>[2x]MATLICGSIAYDNIMTFEGRFREHI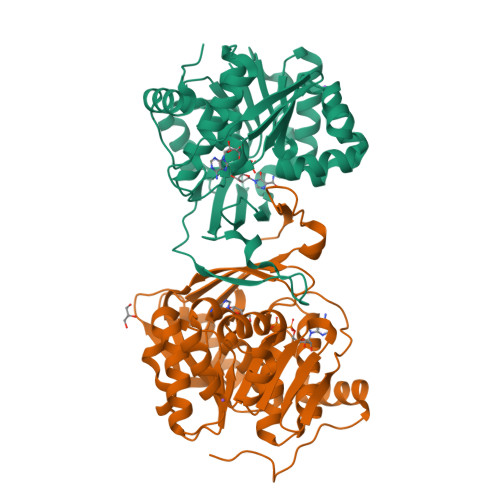LPDQVHLINLSFLVPTMRREFGGCAGNIAYALNLLGGDARMMGTLGAVDAQPYLDRMDALGLSREYVRVLPDTYSAQAMITTDLDNNQITAFHPGAMMQSHVNHAGEAKDIKLAIVGPDGFQGMVQHTEELAQAGVPFIFDPGQGLPLFDGATLRRSIELATYIAVNDYEAKLVCDKTGWSEDEIASRVQALIITRGEHGATIRHRDGTEQIPAVRAERVIDPTGCGDAFRGGLLYGIEHGFDWATAGRLASLMGALKIAHQGPQTYAPTRAEIDARFETAFGYRPKGSKLRSLEHHHHHH>[4x]DIFNRDPRDHYDLLQRLGGGTYGEVFKARDKVSGDLVALKMVKMEPDDDVSTLQKEILILKTCRHANIVAYHGSYLWLQKLWICMEFCGAGSLQDIYQVTGSLSELQISYVCREVLQGLAYLHSQKKIHRDIKGANILINDAGEVRLADFGISAQIGATLARRLAFIGTPYWMAPEVAAVALKGCYNELCDIWSLGITAIELAELQPPLFDVHPLRVLFLMTKSGYQ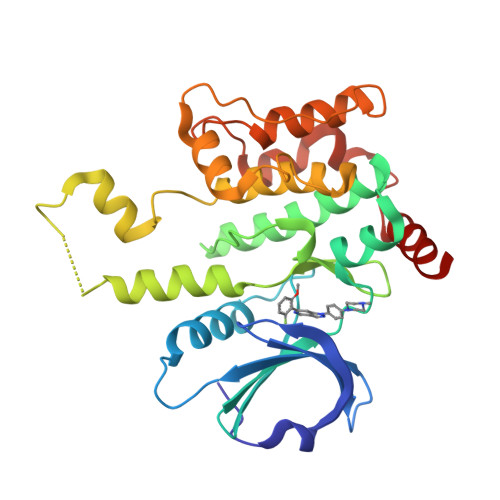PPRLKEKGKWSAAFHNFIKVTLTKSPKKRPSATKMLSHQLVSQPGLNRGLILDLLDKLKNP The adaptor protein paxillin contains five conserved leucine-rich (LD) motifs that interact with a variety of focal adhesion proteins, such as α-parvin. α-parvin (Olski et al., 2001), also known as actopaxin or CH-ILKBP (Tu et al., 2001), is part of the ILK signaling complex (Tu et al., 2001), plays an essential role in adhesion-dependent PKB/Act activation (Fukuda et al., 2003) and in the regulation of actin organization (LaLonde et al., 2005) and Rac activation (LaLonde et al., 2005; Zhang et al., 2004). It belongs to the highly conserved parvin family that shares a common architecture composed of a variable N-terminal region followed by two CH domains (Olski et al., 2001). Our results demonstrate that full-length α-parvin contains a single LD binding site, formed by the N-linker helix, helix A, and helix G of the C-terminal type-5 CH domain.

However, limited proteolysis led to the identification of a stable fragment, α-parvin-CHC, that readily crystallized. This fragment includes residues 242–372 and thereby spans the entire C-terminal CH domain as defined by SMART (Schultz et al., 1998) and a portion of the inter-CH domain linker. The crystal structure of α-parvin-CHC at 1.05 Å resolution was determined by molecular replacement using an ensemble of homologous type-1 CH domain structures as search model. The refined structural model includes α-parvin residues 246–372 (molecule A) or 247–372 (molecule B) and represents the first high-resolution crystal structure of a type-5 CH domain. In spite of very low levels of sequence conservation (≤26% identity) compared to canonical type-1 CH domains, α-parvin-CHC exhibits a typical CH domain core composed of four main α-helices (αA, αC, αE, and αG; nomenclature from Djinovic Carugo et al., 1997), which are connected by loops and shorter helical elements (αD and αF). Atypically, however, the N-terminal boundary of α-parvin-CHC is extended by a short α-helix comprising residues 249 to 256. This “N-linker helix” tightly associates with helices A and G of the canonical CH domain through electrostatic interactions (of residues D248, D251, and D255 with K355 and R359 in αG) and hydrophobic contacts (of residues F250, L253, and F254 with L354, K355, L358, and R359 of αG and K260 and L261 of αA). We therefore conclude that the N-linker helix forms an integral part of the type-5 CH domain of α-parvin, which is in agreement with its resistance to proteolysis. Another feature peculiar to this type-5 CH domain is the loop between helices C and E, which contains a 3 (or 4)-residue insertion (relative to type-1 CH domains) that is conserved throughout the parvin family. Interestingly, the crystal structure of α−parvin-CHC presented here shows that part of the putative ABS2 region is obstructed by the N-linker helix.

>[2x]SGRHERDAFDTLFDHAPDKLNVVKKTLITFVNKHLNKLNLEVTELETQFADGVYLVLLMGLLEGYFVPLHSFFLTPDSFEQKVLNVSFAFELMQDGGLEKPKPRPEDIVNCDLKSTLRVLYNLFTKYRNVE>MKMLLIHSDYLEFEAKEKTKIAEETENLKGKLDECLACFIAVEREDENNPEGTAIGAVEEIEKVANQ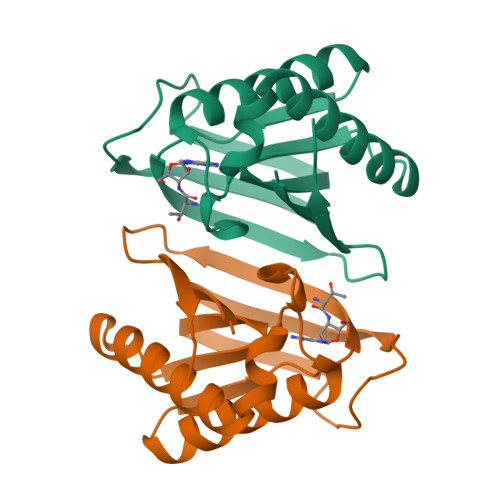LKVNNIVVYPYAHLSSDLSSPETAVKVLKDIESILKERGYNVLRAPFGWYKAFKISCKGHPLSELSRKIVAKEE[4x]>[2x]MPIAVGMIETRGFPAVVEAADAMVKAARVTLVGYEKIGSGRVTVIVRGDVS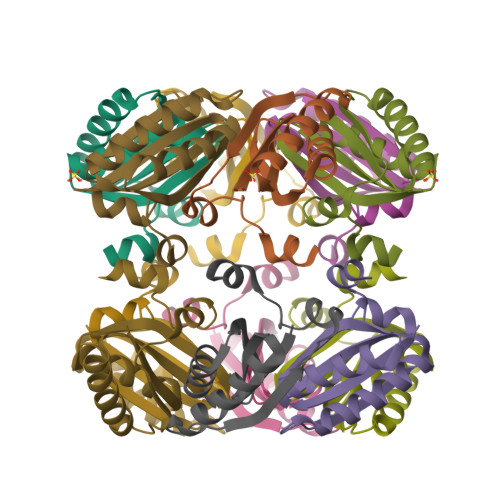EVQASVAAGVDSAKRVNGGEVLSTHIIARPHENLEYVLPIRYTEAVEQFRNLEHHHHHH>MEEEIVKEYM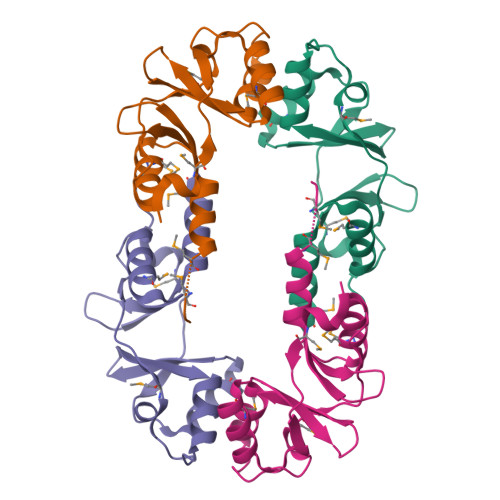KTQVISVTKDAKLNDIAKVMTEKNIGSVIVVDGNKPVGIITERDIVKAIGKGKSLETKAEEFMTASLITIREDSPITGALALMRQFNIRHLPVVDDKGNLKGIISIRDITRAIDDMFETMGEY[2x]NORVALINE | C5 H11 N O2 | 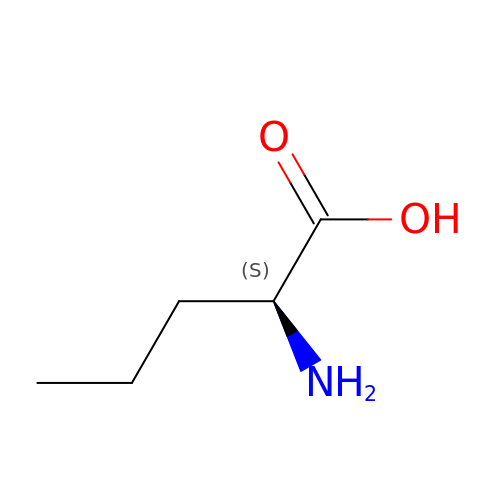SNDPXSYFESPGGJ-BYPYZUCNSA-N PROPANE-1,3-DIYLBIS(PHOSPHONIC ACID) | C3 H10 O6 P2 | 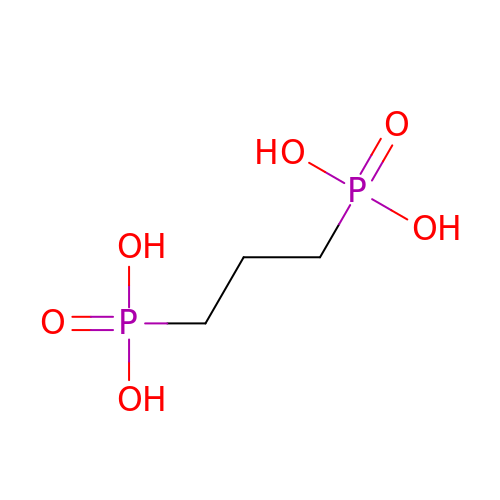PUVMVPFLXCHEOY-UHFFFAOYSA-N N-ACETYL-N-[1-(1,1'-BIPHENYL-4-YLMETHYL)-2-OXOAZEPAN-3-YL]-3-FORMYL-O-PHOSPHONOTYROSINAMIDE | C31 H34 N3 O8 P | 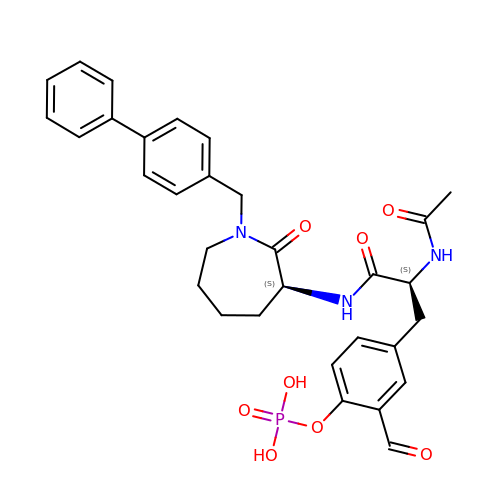SAFPHFWYRLLBFO-NSOVKSMOSA-N> MKKLKKMEQNKTAATRYRQKKRAEQEALTGECKELEKKNEALKERADSL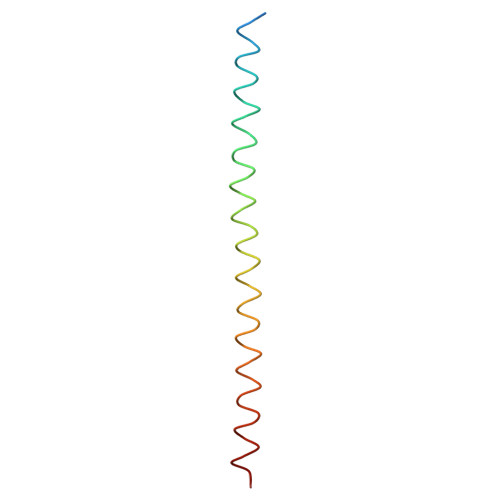AKEIQYLKDLIEEV> MHHHHHHKNIVNTSILSIVYKKDDLIDLSRYGAKINIGDRVYYDSIDKNQIKLINLESSTIEVILKNAIVYNSMYENFSTSFWIKIPKYFSKINLNNEYTIINCIENNSGWKVSLNYGEIIWTLQDNKQNIQRVVFKYSQMVNISDYINRWMFVTITNNRLTKSKIYINGRLIDQKPISNLGNIHASNKIMFKLDGCRDPRRYIMIKYFNLFDKELNEKEIKDLYDSQSNPGILKDFWGNYLQYDKPYYMLNLFDPNKYVDVNNIGIRGYMYLKGPRGSVMTTNIYLNSTLYMGTKFIIKKYASGNEDNIVRNNDRVYINVVVKNKEYRLATNASQAGVEKILSALEIPDVGNLSQVVVMKSKDDQGIRNKCKMNLQDNNGNDIGFVGFHLYDNIAKLVASNWYNRQVGKASRTFGCSWEFIPVDDGWGESSL

The majority of botulinum neurotoxin (BoNT) serotypes require recognition of both the protein and the ganglioside receptor to gain entry in to the cell.

Here, we show that the cell binding domain of BoNT A3 binds three monosaccharides of GD1a receptor. Six residues of the protein interact with this receptor through several key hydrogen bonding interactions.>GIHHVSIKDVLSKYVQLLPNGSSEFRVVKEKDGSSEILTENQVTFDTKTTSEGLVEVTAKFSPNYSLEDGARYVLKFTVTSSQEALDAIAGDKKLEAGDAEGSDVNKLYSNKGASVTYSYGIGNSQTKTKEYSDNPTFKPSDPLTVPVEVEWQGVTGARTVITADQPSNVELKLVQKNKNGGSDNQDYRKTNVNVSKNVSNETRNFEKVAKGYQYDLIAPDVPAFTKEIKNVGTESNPSFKVIYKQLPSLTIKKVLEAENNLNKEFRIKVKLTSPDSKPLNGTFGEITVVNGEAEIRVEKRKRWRGILSYLPRGTHYKVEEEAASTNGYHVTYENQEGDLNKDETSTVTNHKLPSLSVTKKVTGVFANLLKSFKITINIRDAQNSPLNGTYTATVNNKRTPLQFTNGRASIDLNKDQTIKIDGLPLDSH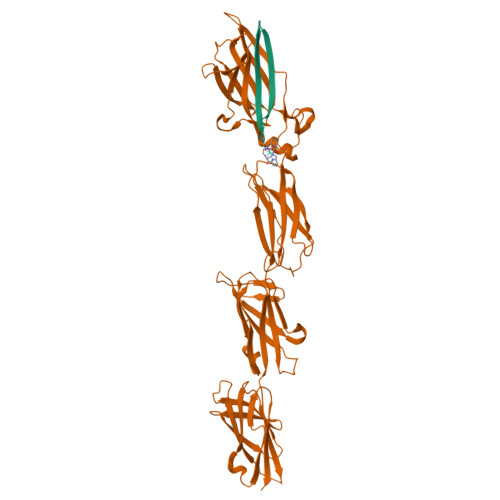YTVEEETNSSRGYQVSYENQEGKLDGDKSATVTNNKNSVPET[2x];>[2x]EPQTTLHKTITPISGQDDKYELSLDITSKL>[2x]MKLTGKQTWVFEHPIFVNSAGTA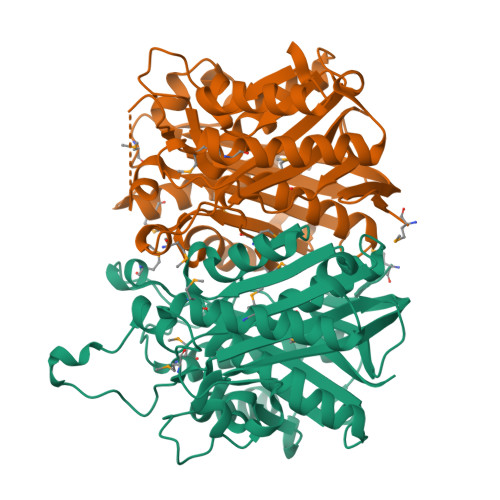AGPKEKDGPLGSLFDKTYDEMHCNQKSWEMAERQLMEDAVNVALQKNNLTKDDIDLLLAGDLLNQNVTANYVARHLKIPFLCMFGACSTSMETVAVASALVDGGFAKRALAATSSHNATAERQFRYPTEYGGQKPDTATSTVTGSGAVVISQTPGDIQITSATVGKVSDLGITDPFDMGSAMAPAAADTIKQHFKDLNRTADDYDLILTGDLSGVGSPIVKDILKEDGYPVGTKHDDCGLLIYTPDQQVFAGGSGCACSAVVTYSHIFKQLREGKLNRVFVVATGALLSPTMIQQKETIPTIAHGVVFERAGGASLEHHHHHH>MAHHHHHHVDDDDKMVHHDGFQTVKATIDWEHPMFKLYEKAKRNGKWNPADIDFSQDQKDFASLTSEEKISALPLVAGFSAGEEAITLDILPMAHALARQGRLEDVLFLTTFMHDEAKHVEMFSRWQQAVGIGQMDLSVFHNDHYKRIFYEALPEAMNRLYADDSPEAVIRAATVYNMIVEGTLAESGYYTFRQIYKKAGLFPGLLQGIDYLNMDEGRHIQFGIYTIQRIVNEDERYYELFIRYMDELWPHVIGYVDYLTEL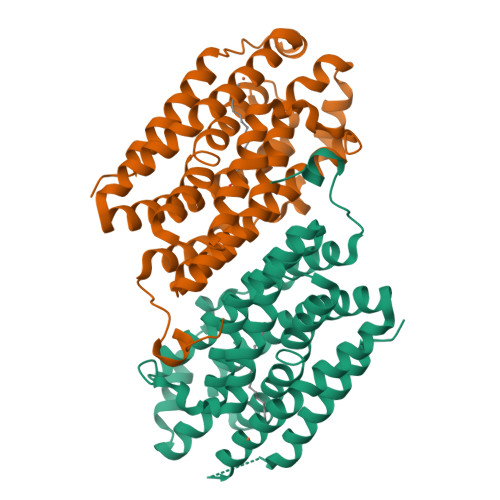GKRQQQLARTYALEIDYDLLRHYVIKQFNLRKKQISRTKRVDVVEGLEKTAAES[2x]>MDEYKTNFIDLTREALSLILQDLKNNVIPKIPVGIEKRERYKNSLRLCLKSARNTQHMNELEPYLELFSECIKNSKLPSHMSLKDQLFYLDKLLENLYFQGVE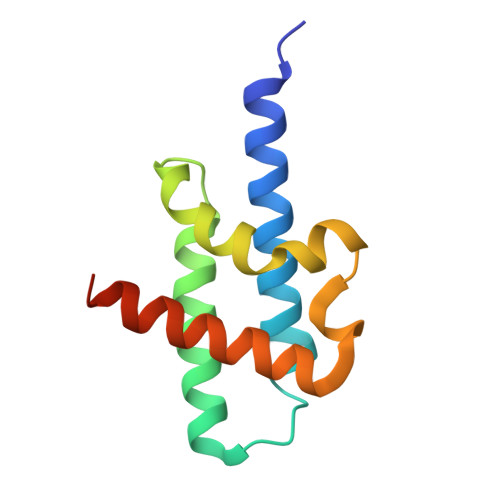HHHHHH[2x]>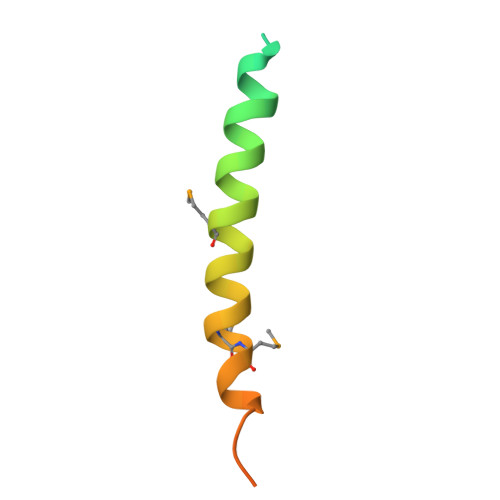 DSSQFADDSGFFDDSEISSIGYEIGSKLAAMCDDFDAQMMSYSAHASDRSLFHRLLD> GPGFDFAQAIMKKNTVVARTEKGEFTMLGVHDRVAVIPTHASVGE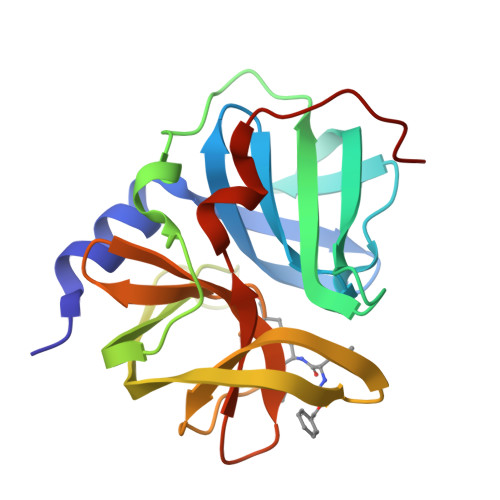TIYINDVETKVLDACALRDLTDTNLEITIVKLDRNQKFRDIRHFLPRYEDDYNDAVLSVHTSKFPNMYIPVGQVTNYGFLNLGGTPTHRILMYNFPTRAGQCGGVVTTTGKVIGIHVGGNGAQGFAAMLLHSYFTDTAKHHHHHH>WSHPQFEKIEGRMSDGRESFLEVMRSVYERYLVGVPGVSEVWLIRHADSYTGLEDYDGDPRDPALSEKGRAQARLLAARLAGVPLHGVWASGAHRAQQTASAVAAEHGLRVRTDARLREVRTNWDDGRPSELKPHGVYPFPEPEKEVAERMRTAVTAAVAATPPAPDGTTRVAVVGHDSALVILMGSLMNLGWGQLDMILPLTSVSVLAVKDERMVVRSIGDATHLAAAPSDVI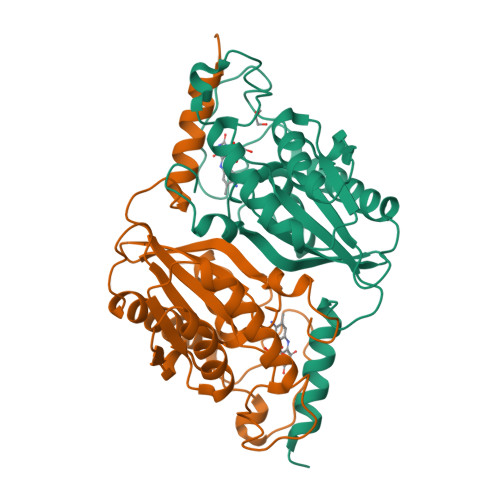[2x]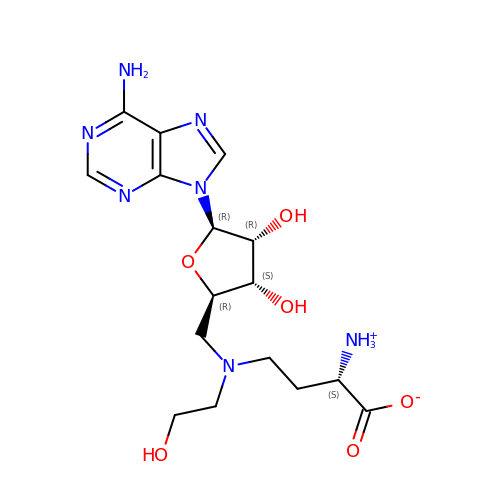(2~{S})-4-[[(2~{R},3~{S},4~{R},5~{R})-5-(6-aminopurin-9-yl)-3,4-bis(oxidanyl)oxolan-2-yl]methyl-(2-hydroxyethyl)amino]-2-azaniumyl-butanoate | C16 H25 N7 O6 | OHBJWDDPDJOYBP-OPYVMVOTSA-N>[2x]MARKYFVAANWKCNGTLESIKSLTNSFNNLDFDPSKLDVVVFPVSVHYDHTRKLLQSKFSTGIQNVSKFGNGSYSGEVSAEIAKDLNIEY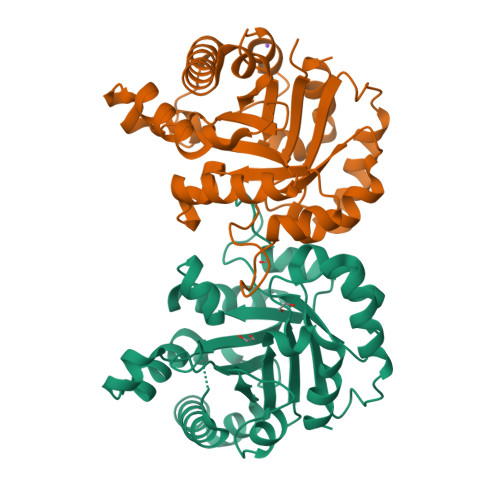VIIGHFERRKYFHETDEDVREKLQASLKNNLKAVVCFGESLEQREQNKTIEVITKQVKAFVDLIDNFDNVILVYEPLWAIGTGKTATPEQAQLVHKEIRKIVKDTCGEKQANQIRILYGGSVNTENCSSLIQQEDIDGFLVGNASLKESFVDIIKSAM> GSNLSELDRL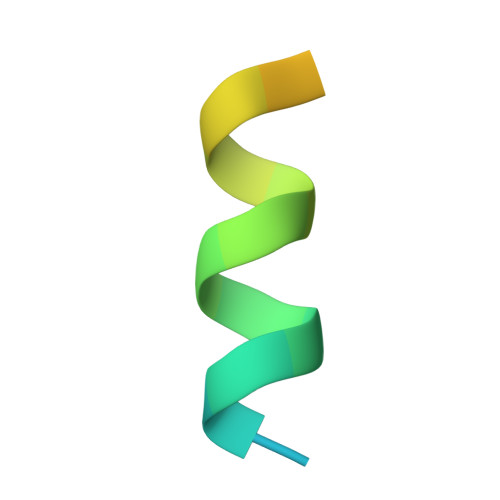LLELNAVQHNPPSG>[2x]SEAEYSPAFALAVGYFKNFIFPAITQIKENGEVNPKICIYKPKHFDELTSTN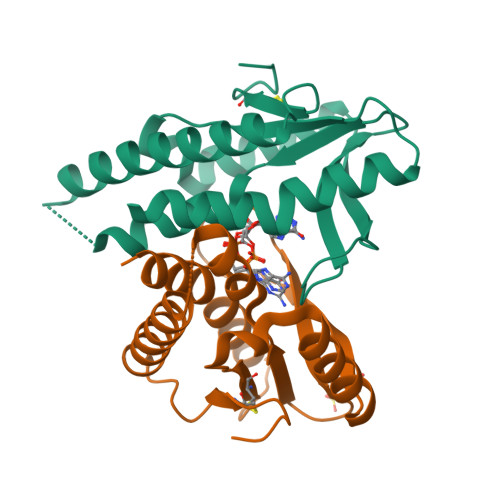IDMIKAELTNKKYNLSEINLSLKGARARDILTLNKKSKIHSYFDFPNTLLSLYSYVDFKIASSNNNSSELKKKKFVELLIEQFYLKLNELIQENNLTNNITFCDKNLQGL> HADPICNKPCKTHDDCSGAWFCQACWNSARTCGP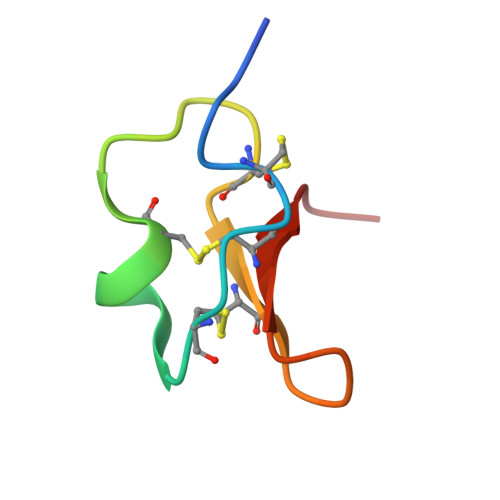YV methyl (2E)-3-methoxy-2-[2-({[6-methyl-3-(trifluoromethyl)quinoxalin-2-yl]oxy}methyl)phenyl]prop-2-enoate | C22 H19 F3 N2 O4 | 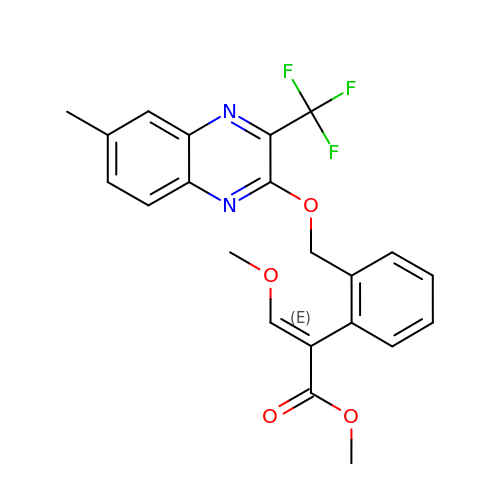GJLNLJPTCNQCFH-FOWTUZBSSA-N The human SSSCA1 gene is located on chromosome 11 (11q13.1) and encodes a small soluble protein of 21.5 kDa with a predicted N- terminal zinc ribbon domain type 2 (ZNRD2), and an unknown domain in the C terminus. We describe the general domain organization of SSSCA1 and identify three distinct domains including an N-terminal zinc finger domain, a disordered region and a C-terminal domain and describe that this domain organization is found in most eukaryotes and is highly conserved. The C-terminal domain has a dual function as we here show the inclusion of an unusual nuclear export signal (NES) that overlaps with a docking site to the poly-ADP-ribosyltransferase Tankyrase 1 (TNKS1). Functionally, SSSCA1 is largely uncharacterized although it has been linked to mitosis and centromere association.

Human SSSCA1 N-terminal Auto_anti-p27 domain (residues 1–111, predicted MW 12.5 kDa) was successfully overexpressed in E. coli and purified over a Ni2+-affinity and size-exclusion chromatography (SEC). The purified SSSCA1 construct was predicted to form a dimer based on the elution time when compared with a set of common standard proteins after SEC (estimated native MW of 24.6 kDa). The crystal structure of N-terminal SSSCA1 was determined at 2.3 Å resolution and phased using the single-wavelength anomalous dispersion method, based on the anomalous signals of two zinc ions. The asymmetric unit contains two protomers that form an antiparallel dimer with a buried surface area of 1960 Å2 (‘Protein interfaces, surfaces, and assemblies’ service PISA35), the interface is highly positively charged and is mainly formed by the helical part of the molecule. Each protomer binds one zinc ion coordinated by four conserved cysteines (human residues Cys53, Cys56, Cys70, and Cys73) structured around four antiparallel β-sheets. We were not able to model residues 1–12 and 78–111 in the electron density map and coincidentally, these regions correlate with the intrinsic disorder prediction plot of SSSCA1 and confirm that these residues likely are disordered in the protein crystal as well. A systematic search for other proteins of similar architecture using available online services, the DALI server, PDBefold37 revealed that SSSCA1 likely belongs to a novel Pfam family of Zn-binding ribbon domains (Auto_anti-p27, PF06677) which overall fold is not yet available in the protein data bank (PDB). The helical dimer interface has not been observed earlier for this type of Zn-binding proteins and the closest zinc-binding protein relative from the zinc ribbon domain 1 family (ZNRD1) do not share this. We have determined the structure of this Cys4 zinc-binding domain and discovered that it belongs to a new family of undescribed zinc-binding proteins denominated Auto_anti-p27 (Pfam PF06677).

>[2x]MALNGAEVDDFSWEPPTEAETKVLQARRERQDRISRLMGDYLLRGYRMLGETCADCGTILLQDKQRKIYCVACQELDSDVDKDNPALNAQAALSQAREHQLASASELPLGSRPAPQPPVPRPEHCEGAAAGLKAAQGPPAPAVPPNTDVMACTQTALLQKLTWASAELGSSTSLETSIQLCGLIRACAEALRSLQQLQH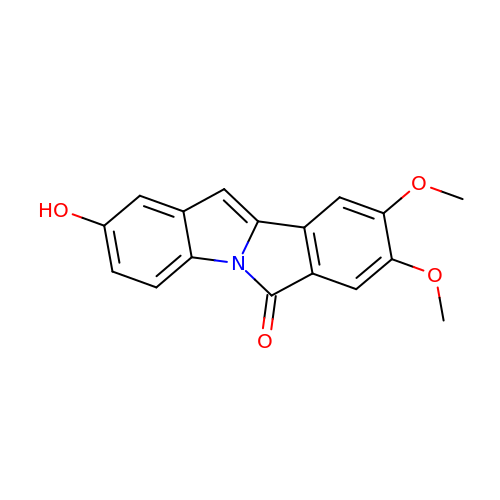2-hydroxy-8,9-dimethoxy-6H-isoindolo[2,1-a]indol-6-one | C17 H13 N O4 | IRPIYZBBHNVOHO-UHFFFAOYSA-N> FACKTANGTAIPIGGGSANVYVNLAPAVNVGQNLVVDLSTQIFCHNDYPETITDYVTLQRGSAYGGVLSSFSGTVKYNGSSYPFPTTSETPRVVYNSRTDKPWPVALYLTPVSSAGGV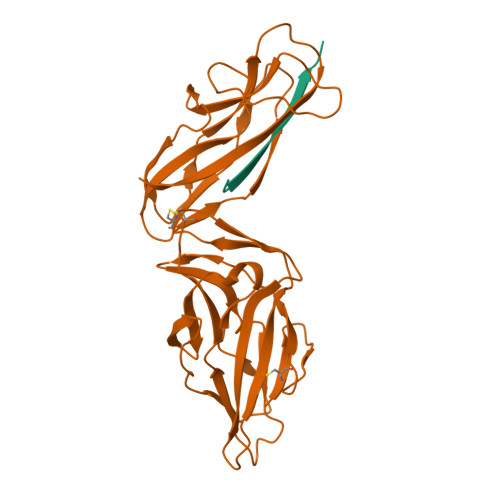AIKAGSLIAVLILRQTNNYNSDDFQFVWNIYANNDVVVPTGGCDVSARDVTVTLPDYPGSVPIPLTVYCAKSQNLGYYLSGTTADAGNSIFTNTASFSPAQGVGVQLTRNGTIIPANNTVSLGAVGTSAVSLGLTANYARTGGQVTAGNVQSIIGVTFVYQ;> ADVTITVNGKVVAK>MPMTVITLKNVPQSLRGDLTRWMQEIATGVYVGNFNSRIREYLWRRVQE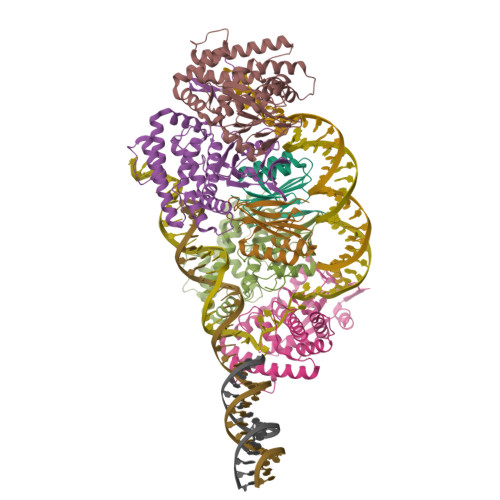TMGAGEASMCFAARNELGYDFLTENASRSVIDYDGLPLIFIPKEQSAVSDLPKGFSTAAKLHRAHIAGSGKKKEKPIRYVVIDIETDGKDAKRNHILEIGAIRCEDGKETHFTALISGDAVPPSITKLTGITATLLQKEGQEEKKVLTAFREFIGDDDLVGYHVSFDIEFLRQAFKKYGLGYLKNKTHDLLRIVKKEQLFQADYKLETSLQSYGIHKKVPHRALGDAELVKCLAKKLNKF[2x];>[4x]MAGPIIAGKSESSELPRVEDRATFIYIEHAKINRVDSAVTVAEAKGVVRIPAAMIGVLLLGPGTDISHRAVELLGDTGTALVWVGEQGVRYYASGRALARSTRFLVKQAELVTNERSRLRVARRMYQMRFPTEDVSKLTMQQLRSHEGARVRRKYRELSKKYNVPWKKRVYNPDDFAGGDPINQALSAAHVALYGLVHSVVAALGLSPGLGFVHTGHDRSFIYDVADLYKAEITVPIAFAVAAEAEEGQDIGQLARLRTRDAFVDGKILKRMVKDLQTLLEIPEEGQIEAEPLSLWDDKEKLVPYGVNYSEVTSCP(5S)-4-[(3E,7E)-4,8-dimethyl-10-(2,6,6-trimethylcyclohex-1-en-1-yl)deca-3,7-dien-1-yl]-5-hydroxyfuran-2(5H)-one | C25 H38 O3 | 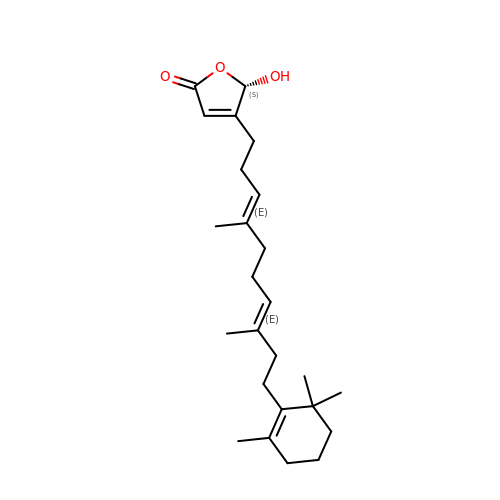JPWPYTMXSXYUPG-XKILHPSWSA-N(2~{R},4~{R},5~{R},6~{R})-2-[(2~{R},4~{R},5~{R},6~{R})-5-[(2~{S},4~{R},5~{R},6~{R})-4-[(2~{R},3~{R},4~{R},5~{S},6~{S})-3-acetamido-6-carboxy-4,5-bis(oxidanyl)oxan-2-yl]oxy-6-[(1~{R})-1,2-bis(oxidanyl)ethyl]-2-carboxy-5-oxidanyl-oxan-2-yl]oxy-6-[(1~{R})-1,2-bis(oxidanyl)ethyl]-2-carboxy-2-[[(2~{R},3~{S},4~{R},5~{R},6~{R})-4-[(3~{S})-3-dodecanoyloxydodecanoyl]oxy-6-[[(2~{R},3~{S},4~{R},5~{R},6~{R})-5-[[(3~{R})-3-heptanoyloxynonanoyl]amino]-3-oxidanyl-4-[(3~{R})-3-oxidanyloctanoyl]oxy-6-phosphonooxy-oxan-2-yl]methoxy]-5-[[(3~{S})-3-[(3~{R})-3-oxidanyldodecanoyl]oxydecanoyl]amino]-3-phosphonooxy-oxan-2-yl]methoxy]oxan-4-yl]oxy-6-[(1~{R})-1,2-bis(oxidanyl)ethyl]-4,5-bis(oxidanyl)oxane-2-carboxylic 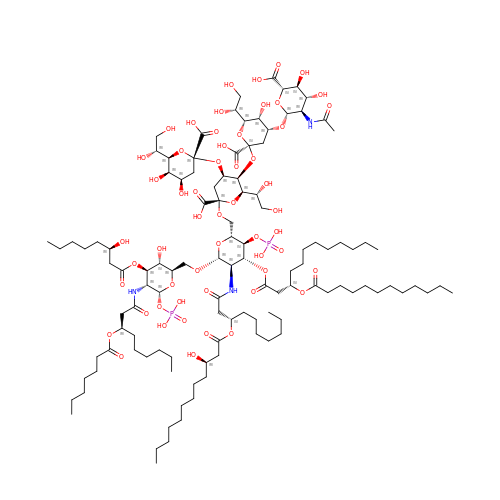acid | C114 H199 N3 O54 P2 | YMSQNHIIBFGVEI-FKAAXFFISA-N> SAHNAYNAGIMQCTGKAFADEFFAEENQVVHESNAVVLVLMKSDEIDAIIEDIVLKGGKAKNPSIVVEDKAGFWWIKADGAIEIDAAEAGELLGK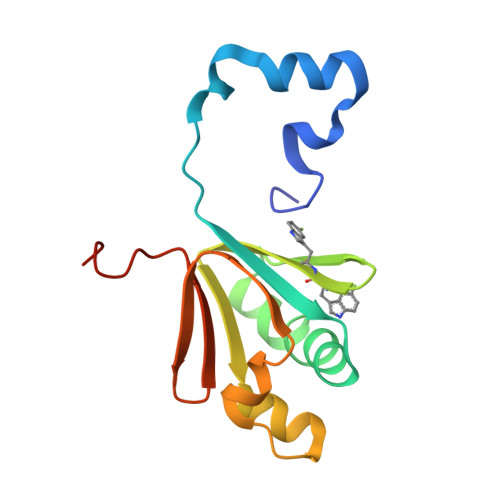PFSVYDLLINVSSTVGRAYTLGTKFTITSELMGLDRALTDI> MNDDRETPPKRKPGEDDTLFDIDFLDDTTSHSGSRSKVTNSHANANYIPPSHVLPEETIDLDADDDNIENDVHENLFMSNNHDDQTSWNANRFDSDAYQPQSLRAVKPPGLFARFGNGLKNAFTFKRKKGPESFEMNHYNAVTNNELDDNYLDSRNKFNIKILFNRYILRKNVGDAEGNGEPRVIHINDSLANSSFGYSDNHISTTKYNFATFLPKFLFQEFSKYANLFFLCTSAIQQVPHVSPTNRYTTIGTLLVVLIVSAMKECIEDIKRANSDKELNNSTAEIFSEAHDDFVEKRWIDIRVGDIIRVKSEEPIPADTIILSSSEPEGLCYIETANLDGETNLKIKQSRVETAKFIDVKTLKNMNGKVVSEQPNSSLYTYEGTMTLNDRQIPLSPDQMILRGATLRNTAWIFGLVIFTGHETKLLRNATATPIKRTAVEKIINRQIIALFTVLIVLILISSIGNVIMSTADAKHLSYLYLEGTNKAGLFFKDFLTFWILFSNLVPISLFVTVELIKYYQAFMIGSDLDLYYEKTDTPTVVRTSSLVEELGQIEYIFSDKTGTLTRNIMEFKSCSIAGHCYDDKIPEDKTATVEDGIEVGYRKFDDLKKKLNDPSDEDSPIINDFLTLLATCHTVIPEFQSDGSIKYQAASPDEGALVQGGADLGYKFIIRKPNSVTVLLEETGEEKEYQLLNICEFNSTRKRMSAIFRFPDGSIKLFCKGADTVILERLDDEANQYVEATMRHLEDYASEGLRTLCLAMRDISEGEYEEWNSIYNEAATTLDNRAEKLDEAANLIEKNLILIGATAIEDKLQDGVPETIHTLQEAGIKIWVLTGDRQETAINIGMSCRLLSEDMNLLIINEETRDDTERNLLEKINALNEHQLSTHDMNTLALVIDGKSLGFALEPELEDYLLTVAKLCKAVICCRVSPLQKALVVKMVKRKSSSLLLAIGDGANDVSMIQAAHVGVGISGMEGMQAARSADIAVGQFKFLKKLLLVHGSWSYQRISVAILYSFYKNTALYMTQFWYVFANAFSGQSIMESWTMSFYNLFFTVWPPFVIGVFDQFVSSRLLERYPQLYKLGQKGQFFSVYIFWGWIINGFFHSAIVFIGTILIYRYGFALNMHGELADHWSWGVTVYTTSVIIVLGKAALVTNQWTKFTLIAIPGSLLFWLIFFPIYASIFPHANISREYYGVVKHTYGSGVFWLTLIVLPIFALVRDFLWKYYKRMYEPETYHVIQEMQKYNISDSRPHVQQFQNAIRKVRQVQRMKKQRGFAFSQAEEGGQEKIVRMYDTTQKRGKYGELQDASANPFNDNNGLGSNDFESAEPFIENPFADGNQNSNRFSSSRDDISFDI;> MVSLFKRGKAPPLTKEGPTSKKPPNTAFRQQRLKAWQPILSPQSVLPLLIFVACIFTPIGIGLIVSATKVQDLTIDYSHCDTKASTTAFEDIPKKYIKYHFKSKVENKPQWRLTENENGEQSCE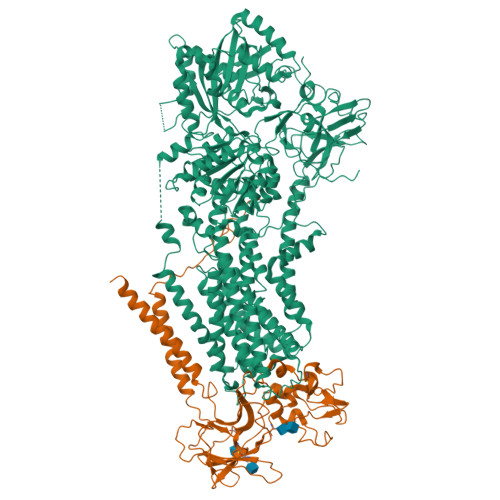LQFEIPNDIKKSIFIYYKITNFYQNHRRYVQSFDTKQILGEPIKKDDLDTSCSPIRSREDKIIYPCGLIANSMFNDTFSQVLSGIDDTEDYNLTNKHISWSIDRHRFKTTKYNASDIVPPPNWMKKYPDGYTDENLPDIHTWEEFQVWMRTAAFPKFYKLTLKNESASLPKGKYQMNIELNYPISLFGGTKSFVLTTNGAIGGRNMSLGVLYLIVAGLCALFGIIFLVKLIFQPRAMGDHTYLNFDDEENEDYEDVHAENTTLREIL> MGSSHHHHHHSSGLVPRGSHMASADFTQGADVSGNNVTLWFKSSVNTTWVDVHYKVNSGVQQNVRMSFNAGAARFEHTILTAAQAEIEYFFTYNNGVPAYDTTTFTYRSGQPDPEPSTNSIYSIPASSIPQPSEGGVSLKVMNGTGGAYTD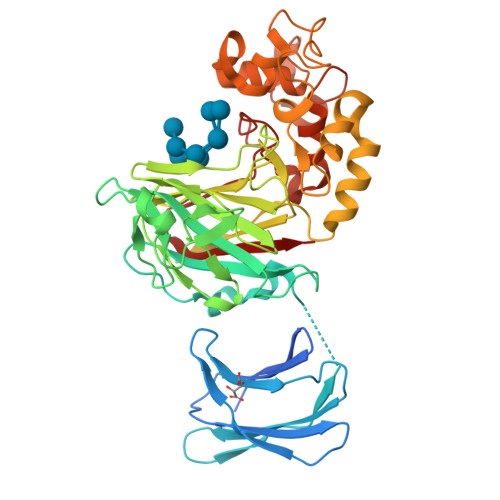DQIYWGVIGINPVNGKWSYLDLAGRLLPISSDLNNAPGHLTKDGINYANIYHKISDANWVNLPKIESGRLFLSVGSPLYMKTFDDGFAGPDLNNPTDPNLNIIFDFVAFTVDKDGYHGNTTRVDQFGFPIQHRLVNLAGNYDRTVGELESETRSGLFAKYVNEVPYEFKSLGTLQAPYRILSPMKGPFQEGGAYENYFAGYSSISTQDILLGVGEASNPEVCAALNRHVYTEPDNWNRVDQYYQAAPANYYAKFWHDHSIDGLAYGFCYDDVNGQAAYLEVGDPKGLIVRVGW>[4x]MGLSLPKEKGLILCLWSKFCRWFQRRESWAQSRDEQNLLQQKRIWESPLLLAAKDNDVQALNKLLKYEDCKVHQRGAMGETALHIAALYDNLEAAMVLMEAAPELVFEPMTSELYEGQTALHIAVVNQNMNLVRALLARRASVSARATGTAFRRSPCNLIYFGEHPLSFAACVNSEEIVRLLIEHGADIRAQDSLGNTVLHILILQPNKTFACQMYNLLLSYDRHGDHLQPLDLVPNHQGLTPFKLAGVEGNTVMFQHLMQKRKHTQWTYGPLTSTLYDLTEIDSSGDEQSLLELIITTKKREARQILDQTPVKELVSLKWKRYGRPYFCMLGAIYLLYIICFTMCCIYRPLKPRTNNRTSPRDNTLLQQKLLQEAYMTPKDDIRLVGELVTVIGAIIILLVEVPDIFRMGVTRFFGQTILGGPFHVLIITYAFMVLVTMVMRLISASGEVVPMSFALVLGWCNVMAFARGFQMLGPFTIMIQKMIFGDLMRFCWLMAVVILGFASAFYIIFQTEDPEELGHFYDYPMALFSTFELFLTIIDGPANYNVDLPFMYSITYAAFAIIATLLMLNLLIAMMGDTHWRVAHERDELWRAQIVATTVMLERKLPRCLWPRSGICGREYGLGDRWFLRVEDRQDLNRQRIQRYAQAFHTRGSEDLDKDSVEKLELGCPFSPHLSLPMPSVSRSTSRSSANWERLRQGTLRRDLRGIINRGLEDGESWEYQILVPRGSAAAWSHPQFEK

TRPV6, a highly calcium-selective TRP channel, is overexpressed in endometrial cancers, leukemia, and carcinomas of the breast, prostate, colon, ovarian, and thyroid. TRPV6 has four subunits that form a transmembrane domain (TMD) with a central ion channel pore, an intracellular skirt domain enclosing a large cavity, and amphipathic TRP helices that run nearly parallel to the membrane and interact with both the TMD and the skirt. The TMD is composed of transmembrane helices S1–S6 and a re-entrant pore loop (P-loop) between S5 and S6. The first four transmembrane helices form a bundle to constitute the S1–S4 domain.

We thus turned to human TRPV6 (hTRPV6), of which we recently resolved the open-state structure by cryo-electron microscopy (cryo-EM). In order to increase the affinity of hTRPV6 to 2-APB, we introduced the Y467A mutation, homologous to Y466A in TRPV6*. As expected, hTRPV6-Y467A showed 4.5-fold increased potency of 2-APB inhibition (IC50 = 60 ± 13 μM, n = 3) compared to hTRPV6. We determined the cryo-EM structure of apo hTRPV6-Y467A, which is in the open-state conformation, and it is nearly identical (RMSD = 0.765) to the cryo-EM structure of wild-type hTRPV6. Lipids are observed in positions similar to those seen in hTRPV641; lipid 1 is bound in a pocket formed by the intracellular half of the S1–S4 domains and C-terminal part of TRP helix, while lipid 2 is above the S4–S5 linker and contacts both S3 and S4 of the same subunit, and S5–S6 of the neighboring subunit. In both hTRPV641 and hTRPV6-Y467A, the activating lipid head penetrates this area to interact with Q483 and R470.>[6x]MTPHINAKIGDFYPQCLLCGDPLRV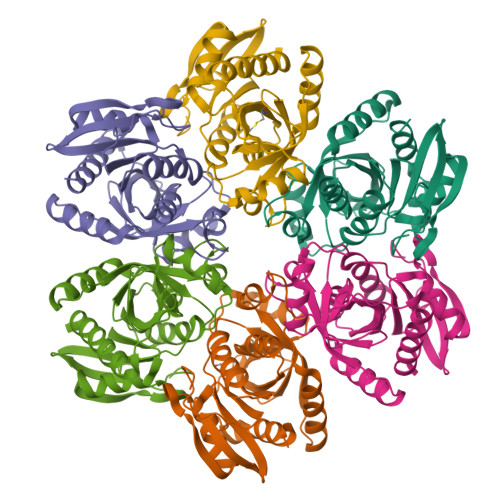SYIAKKFLQDAKEITNVRNMLGFSGKYKGRGISLMGHGMGIASCTIYVTELIKTYQVKELLRIGTCGAISPKVGLKDIIMATGASTDSKTNRVRFLNHDLSATPDFELSLRAYQTAKRLGIDLKVGNVFSSDFFYSFETHAFDLMAKYNHLAIEMEAAGLYATAMELNAKALCLCSVSDHLITKEALSPKERVESFDNMIILALEMMS(3S,3AR,4S,6S,6AR,7S,8S,9BS)-6-(ACETYLOXY)-3,3A-DIHYDROXY-3,6,9-TRIMETHYL-8-{[(2Z)-2-METHYLBUT-2-ENOYL]OXY}-7-(OCTANOYLOXY)-2-OXO-2,3,3A,4,5,6,6A,7,8,9B-DECAHYDROAZULENO[4,5-B]FURAN-4-YL 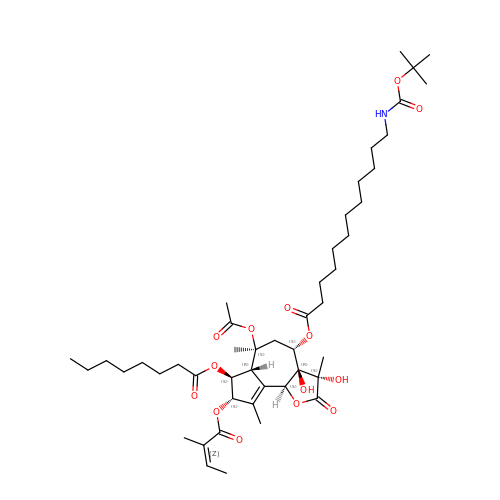12-[(TERT-BUTOXYCARBONYL)AMINO]DODECANOATE | C47 H75 N O14 | IBTNJSDBPZIGKM-GGGDSPQJSA-N> MGSYFVPPANYFFKDIFASNVGNIANVIFDNGNVIAAGGLGYLIGNGAFITGVTSTAIANIPAVVTADIRGNLIGNYANVNNIIASSGNISNVRFVSGGNVTASYYFGDGSQLTGITATANIPSIVTADIRGNIIGNYANVSNVSATFGNIANVLFNNGNVTAAGGNGFFIGNGSLLTGITATANIPSIVTADIRGNIIGNYANVSNVSATFGNIANVLFNNGNVTAAGGNGYFFGNGALLTGITATANIPSIVTADIRGNIIGNYANVSNVSATFGNIANVLFNNGNVTAAGGNGYFFGNGALLTGITATANIPSIVTADIRGNIIGNYANVSNVSATFGNIANVLFNNGNVTAAGGNGFFIGNGSLLSGITATANIPSIVTADIRGNIIGNYANVSNVTATFGNIANVLFNNGNVTAAGGNGYFFGNGSQLTGVTATLPSIVTADIRGNIIGNYANVSNVIATFGNIANVLFNNGNVTAADGNGYFFGNGSQL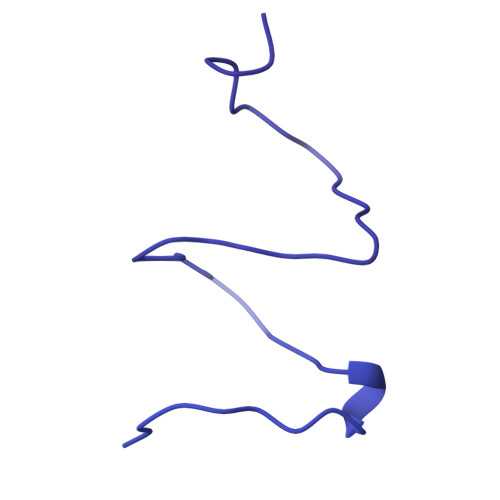TGVTATLPSIVTADIRGNIIGNYANVSNVIATFGNIANVLFNNGNVTAAGGNGYFFGNGALLTGITATANIPSIVTADIRGNIIGNYANVSNVIATFGNIANVLFNNGNVTAADGNGYFFGNGSQLTGVTATLPSIVTADIRGNIIGNYANVSNVIATFGNIANVLFNNGNVTAAGGNGYFFGNGALLTGITATANIPSIVTADIRGNIIGNYANVSNVTATFGNIANVLFNNGNVTAAGGNGYFFGNGSQLTGVTATLPSIVTADIRGNIIGNYANVSNVIATFGNIANVLFNNGNVTAAGGNGYFFGNGALLTGITATANIPSIVTADIRGNIIGNYANVSNVTATFGNIGNVLFNNGNVTAAGGNGYFFGNGTFLNFSTITADIRGNIIGNYANVGNVIAGNVSTTLGNIGNVLFNNGNVTAAGGNGYFFGNGTSLTFSTIRADIRGNIIGNYANVANVIAGNVNSTFGNIAGVTFDAGNVSSPVDILVSGNVSVGSDGLFRGPTNQSNNALILRGIGGTNTVNLFSIGAPSGQMRFSVPASGVAFYNFLYGTNQVASLGPQGFYSLSYDSSVVVGQVVSNSTTYSGTIFKTEANRNSSTAFNHISCTGSNGNVFRVRGDGTTYGVGAFQTSGADYAEMMEWEDKNPTFEDRRGYPVVLSGNGKIRIASLSDDYNNIIGVVSSNPSMLADMAWDQWEGKYLKDKFGMRLSNTIYYLANISNENEFTRVGPMTTPPQGYFIKTSPEYILNPKYNPNVAYVERNDRPEWDPVGFVGKLRVRNGCLVHPSWKPLKVIDDYADVGNAAAQVTEYLIGVTPNYTLSKKVEDLEQTINVLKTQVQMLLGNI> GYQIGEAAQMVTNTKGIQDLSDRYESLNNLLNRYSTLNTLIKLSADPSAINAVRENLGASAKNLIGDKANSPAYQAVLLAINAAVGFWNVVGYVTQCGGNANGQKSISSKTIFNNEPGYRSTSITCSLNGHSPGYYGPMSIENFKKLNEAYQILQTALKRGLPALKENNGKVNVTYTYTCSGDGNNNCSSQVTGVNNQKDGTKTKIQTIDGKSVTTTISSKVVDSRADGNTTGVSYTEITNKLEGVPDSAQALLAQASTLINTINNACPYFHASNSSEANAPKFSTTTGKICGAFSEEISAIQKMITDAQELVNQTSVINEHEQTTPVGNNNGKPFNPFTDASFAQGMLANASAQAKMLNLAEQVGQAINPERLSGTFQNFVKGFLATCNNPSTAGTGGTQGSAPGTVTTQTFASGCAYVGQTITNLKNSIAHFGTQEQQIQQAENIADTLVNFKSRYSELGNTYNSITTALSNIPNAQSLQNAVSKKNNPYSPQGIDTNYYLNQNSYNQIQTINQELKKKKKKGSEQKLISEEDL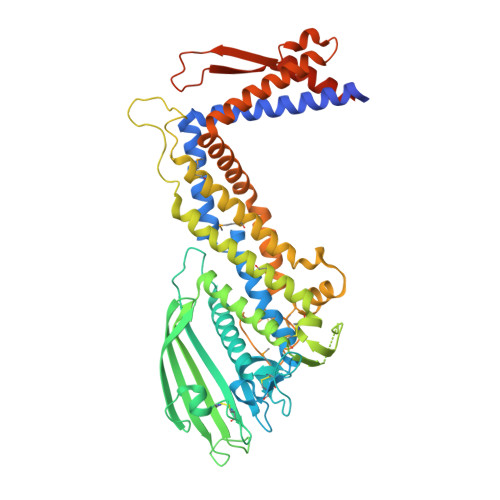SHHHHHH>[2x]MDDISVIKNEDYEGSHRFLAEELLMPNANKTDGNRSTMFCSHLAQAVTLQKAEPPLVYTNFENQVGKYSTAGYRKANSNYKVIEKIYKNDYNYVLIVQDQETGEYTLFERAECEFLTEHYGFQWDNDKIDSLKKDDTIEKDTVLYKNTCYDENMNFGYGVNLNAAYFSYKNETLEDAIVISESAAKKLGTFSVNKVKVSVNTNDILLNLYGDNENYKGFPDIGEHIKNQIIASRRRFDYNTALYELKNLNEMRDSDTPFFADGKIVDIEIFSNVPEEELKVQKYNEQVLYYINKQKEFSNNVYQKLKKIVEGKDNNVSDKLLHFYNNCKMRIDENISYTYQNSKFSGFIMEFTILEEEPLNKGSKITGRYGNKGVISKILPDDQMPTVAEGRFKGLKADICLNPLGVFNRLNPSQLIEQELNWIAKFIRKDMEEAGSNEEKVSILLDFLNRVNKEETELMEEFINSLNKTELEEFLNDIIENGIPICQKPFFGNIGLDELWELYNHYDHIDYFKCEGISTPLIIGEIYMVRLKHEPHSKFSARSTSFMNLRGLPAKSKNFKEHKDLYSKTPVRIGNMEISNLSLTNEMGSIMDMLNSYSNNETNRRELIMQLLTGNPFDTNIDLSDVESGTSKILKSLFTCLGLSIDDVEEEWENKLNGKVEDEK;>MEKTYNLNDILLSNEYEKIKEDIKEEIINDMASKKVKYSNTSEFAKNDFLKDEFIDLVVDGETYEITYGNLITLLIVARPFNHFKVPMTEDLLFDLSDLKEYQNYYTTLLEHFGYSNEIKSIIKDVISELAIFSGDINVTFGNTVSIKSLIDLGNKVKRFRELLHYRLPNDEALEFNDIEAIIKKNLDEIMKILSETDNMLRYYIDSGAGINSKQFGQVLSLVGSKPDLFGKIIPYPINTSFLRGLDVRSFYINALGARKALITNYQQVRNSGYLTRKISMLLMDTKLIDLDDCGSHENNYLSINVENKDVLKRFSKRSYLNNNGELVEIDINDESLIGQVIKIPSPTTCASNEGVCRKCYGKLFDINKDLNIGMIAVLLLTDPLTQRLLSAKHLLETRSSKIDWGTNFEENFIVNRNLIYPKVYNGTVIIKEDDFKEDEETEEQVFDTFTLKSGNRFISISSPMRLFLNKDLKKQLDESFYNIEEMQFEIPLNKLDEGDSFATFIMDNNELSKPLREIKDLIETNKYIKDHNVNEVVNYFIYLLNESGINIQSVHSELIIREMMKLDDSDRTQFKNDKMPDYEIFRITDANLKGDSLSRSLLFEQVKKQLTTLDYDTFNKTKSSILDKLL[2x];>[2x]MISNFRKFHGNKNQEKFNENLILNKENESILNYLDPICKTLEIIPEITYLGSSVEPINKVYKFNKEEKTSDIERSELQLIKMSFLIEKDDKKEEINKFIYFPKLIDSQYFIINGNRYYPIYQLLDSGTYRTNKALTLKTLLMPIVLREKKETFDDINGETHTMLNVDLDLFKSKVPFLIYFFSKFGFEGTLEYFGLQDLIHVLMKEDLDQLDEDEINDNVIFMITKNISLVVDKNFFSNKNNQIIIATLLNCFNTRIKIDKIYEKDYWVKKLGGYFTTNNSNKQEKGEGIILSFERILDEWTKKILRTEEKNKEDIYSVVRWMINNYLALVKQDNMNLANKRIRLYEYLLHPLLIKFSKGTYRVLNNRNSNKFEKIKTIFSNIQEGFLVKKIINNELLRYDNSVNSISLFTLILRYTQSGPQSPFSSNSTNNKLRGLHPSYLGRLGLTSTSAGDPGASGSLTPFL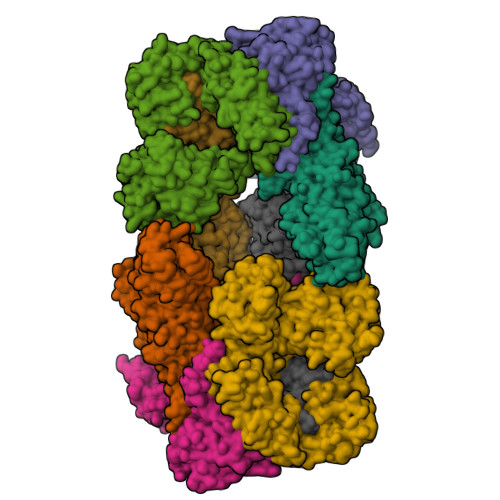ELPENSYMHFTEEPEINLNIDDISIDEVIES;>[2x]MGSSHHHHHHSSGENLYFQGHHMGKKLSLIDFNEIYNEENLITRANPIENHEFSDDGIYSERIFGSYNEDDDDKDIDTIGWINIEPYYIINPILFTIIKKCIPSINKIINYQQSIDQNGENIDLTEEIGEDDYIGLVKFKDNFDDLLEKYTDKKKYQKEYDFLIENHDKIFINKLPVFSHKLRPATLLTGSKGKVLAFDEINNYYNFVIEYINQINEGVVSDDSIDLLLLPLLYNMQFYANNILTRIISEYLRGKKGFLRKNIMGSRINFSARNVITPLIGHPIDEVAMPYKTFAELYKFQLINLISKVKGINYNEALKFWEKGILGFNQELYNYMEELITKTKGGCTFLLNRNPTISIGSILYLKIGLIKKDYKDLTLGISNNLLSALSGDYDGDVLNIIPVFDNKMKEHFSLLSPQNFLVDRNNGRFNGDFDLQKDQILGIFILNN2-[(1~{S})-2-oxidanylidenecyclopentyl]ethanoic 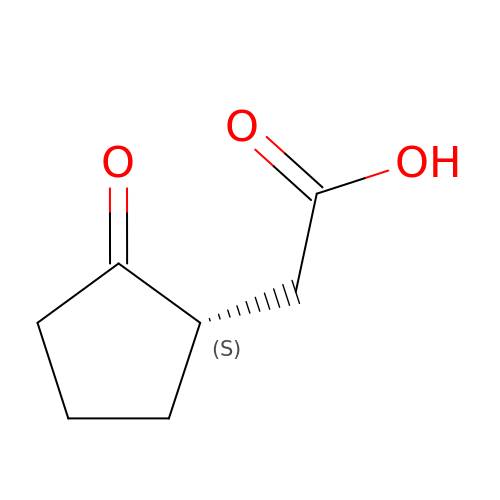acid | C7 H10 O3 | OLLLIBGOZUPLOK-YFKPBYRVSA-N>[6x]MTERTLVLIKPDGIERQLIGEIIS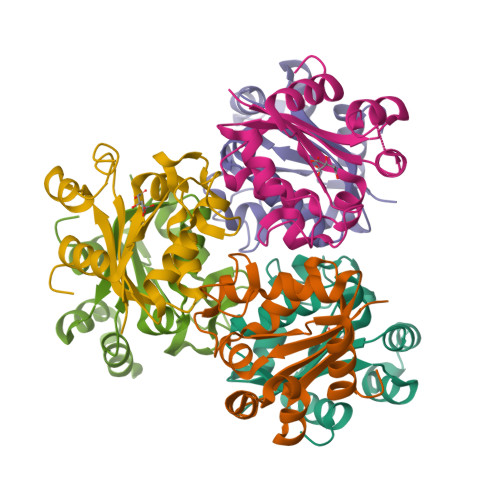RIERKGLTIAALQLRTVSAELASQHYAEHEGKPFFGSLLEFITSGPVVAAIVEGTNAIAAVRQLAGGTDPVQAAAPGTIRGDFALETQFNLVHGSDSAESAQREIALWFPGA Among them, a new esterase PMGL2 belonging to the hormone sensitive lipase (HSL, EC 3.1.1.79) family (family IV lipases) was produced and biochemically characterized. The unique feature of this enzyme is the presence of a cysteine residue in the GCSAG motif which surrounds the conserved catalytic serine. Three-dimensional structures of subunits of wtPMGL2 and its mutant variant mPMGL2 were found to be quite similar (see Methods section). Both of them had a typical α/β bacterial HSL-like fold, consisting of two canonical domains ‒ a CAP-domain and a catalytic domain. The active site of PMGL2 consists of a catalytic triad of conserved His302, Asp272 and Ser174.

To unravel the effect of the unusual Cys173 on the properties of wtPMGL2, two point mutations were introduced in positions C173T and C202S resulting in mPMGL2 mutant variant. In accordance with biochemical data, the structural analysis of mPMGL2 didn’t reveal any dramatic structural changes either, neither in the active site cavity nor in an overall fold of mPMGL2 in comparison with wtPMGL2. While Thr173 wasn’t forming any hydrogen bonds to the adjacent residues (except for the solvent molecule), the side chain of Ser202 participated in two new hydrogen bonds, one to a nitrogen atom of Ala303 and another one to OD2 atom of catalytic Asp272. For unknown reasons, despite the same conformation of the loops 202–209 and 216–237 in both wtPMGL2 and mPMGL2 structures, a PEG molecule was found only in the active site of mPGML2. Each subunit of the asymmetric unit contains one PEG molecule bound in the active site cavity mainly via hydrophobic interactions. Key residues which participate in the cavity formation are: Thr204 and Ala206 which anchor PEG molecule by hydrogen bonds to its oxygen via their main chain, Gly107-Phe109, Thr173-Gly176, Val178, Ser202-Tyr208, Val218, Leu234-Thr236 and Asp272-Ala274. In the B subunit of mPMGL2, the PEG molecule was found in two conformations. The presence of two different PEG molecule conformations in the active site cavity most likely resulted from inefficient binding of this substrate analogue. In contrast to wtPMGL2, in mPMGL2 the Tyr208 has one distinct conformation, resembling the one from the structure of wtPMGL2, which allows binding of the PEG molecule in the active site. Interestingly, PEG molecule was found in the active site of mPMGL2 (but not in wtPMGL2). This finding makes mPMGL2 structure a unique example of family IV lipases with a bound ligand analogue, besides known structures with small inhibitors like PMSF.

>[2x]MASGSASSAQTPGLMSWLPPSNQLSPEARSVLDRMDAAKAPEFNGDLVRQRAFYQQFNDDRLVEMRRVFRTRERHETLNAVHVQVVEPADGVSARNRDRVLINVHGGAFMWGAGSGALVEAIPIAATMGVSVVTVDYRLAPENRYPAASEDVTAVYRALLERYPAANIGIFGTSAGGVITAQAVTWIRREGLPRPGAIGTLSGTGAPYSGDSPYLAGVVPVGPGVKAPPLPGLLPTAYMEGVGADDARAYPLTSDAETVFMPPTLLLAGGRDFAVSALSLAHRRLARAGVDSELHLFDGLPHAFFVWPDMPESLEAYALIAGFFDSRLGLTPSSSIPTPRSPSLEHHHHHH>SKVKVAVRIRPMNRRETD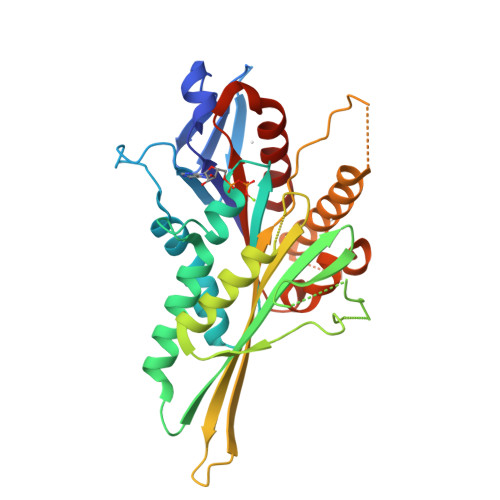LHTKCVVDVDANKVILNPVNTNLSKGDARGQPKVFAYDHCFWSMDESVKEKYAGQDIVFKCLGENILQNAFDGYNACIFAYGQTGSGKSYTMMGTADQPGLIPRLCSGLFERTQKEENEEQSFKVEVSYMEIYNEKVRDLLDPKGSRQTLKVREHSVLGPYVDGLSKLAVTSYKDIESLMSEGNKSRTVAATNMNEESSRSHAVFKITLTHTLYDVKSGTSGEKVGKLSLVDLAGSERATKTGAAGDRLKEGSNINKSLTTLGLVISALADQSAGKNKNKFVPYRDSVLTWLLKDSLGGNSKTAMVATVSPAADNYDETLSTLRYADRAKHHHHHH[3x]The potassium ion efflux channel GORK plays a critical role in closing plant leaf stomata by releasing K+ from guard cells to reduce guard cell volume and turgor. The GUARD CELL OUTWARD-RECTIFYING K+ (GORK) channel is expressed in Arabidopsis guard cells and encodes a K+out channel. Voltage-dependent K+ channels, including GORK, contain three regions: an intracellular N-terminal region, a transmembrane region, and an intracellular C-terminal region (27–30). The transmembrane region is composed of six transmembrane helices (S1-S6), with S1-S4 forming the voltage sensing domain and S5 and S6 forming the pore region.

As a result, five different structures of GORK ranging from the transmembrane region to the C-terminal ANK (designated as GORKWT1–GORKWT5) were determined at resolutions of 3.16 to 3.27 Å. The five GORK structures showed N-terminally an almost uniform transmembrane domain (positions 50 to 313 from the initial Met), including the voltage-sensing domain and the ion selectivity filter. In contrast, the following cytosolic regions, i.e., C-linker (positions 314 to 364), CNBD (positions 365 to 490), CNBD–Ankyrin bridge (positions 491 to 542), and ANK (positions 543 to 722) show five distinct structures in almost twofold symmetry (C2 symmetry). Furthermore, overlaying GORKWT1 and GORKWT5, which had high resolutions of 3.17 and 3.16 Å, respectively, revealed that one of the C-linkers in each dimer was pushed upward by the CNBD in GORKWT1, as compared to GORKWT5. Closer inspection of the structure revealed that the difference of the degree of bending in the C-linker between Mol I and Mol II was small in GORKWT1 but greater in GORKWT5. Additionally, GORKWT1 displayed a C4-like C2 symmetry in the CNBD, whereas GORKWT5 showed a pronounced C2 symmetry. Furthermore, we found a structural difference in the short structure that lies between the CNBD and ANK domains, termed as CNBD–Ankyrin bridge containing residues 511 to 519. This region had an α-helical structure in GORKWT1, while in GORKWT5, it was entirely present in a nonhelical loop conformation. The CNBD–Ankyrin bridges of GORKWT1–GORKWT5 contain a mixture of α-helical and nonhelical structures, and these conformational changes appear to be centered around L516.

>MDYKDDDDKGRLRRRQEIIDHEEEESNDDVSSRRGKLSLAETFRWLDSSEHRRIETDGHNDYKYIIHPKNRWYKAWEMFILVWAIYSSLFTPMEFGFFRGLPERLFVLDIVGQIAFLVDIVLQFFVAYRDTQTYRTVYKPTRIAFRYLKSHFLMDFIGCFPWDLIYKASGKHELVRYLLWIRLFRVRKVVEFFQRLEKDTRINYLFTRILKLLFVEVYCTHTAACIFYYLATTLPPENEGYTWIGSLKLGDYSYENFREIDLWKRYTTALYFAIVTMATVGYGDIHAVNLREMIFVMIYVSFDMVLGAYLIGNITALIVKGSNTERFRDKMNDLISFMNRKKLGRDLRSQITGHVRLQYDSHYTDTVMLQDIPASIRAKIAQLLYLPYIKKVPLFKGCSTEFINQIVIRLHEEYFLPGEVITEQGNVVDHLYFVCEGLLEALVTKTDGSEESVTLLGPHTSFGDISIICNISQPFTVRVCELCHLLRLDKQSFSNILEIYFHDGRTILNNIMEEKESNDRIKKLESDIVIHIGKQEAELALKVNSAAFQGDFYQLKSLIRSGADPNKTDYDGRSPLHLAACRGYEDITLFLIQEGVDVNLKDKFGHTPLFEAVKAGQEGVIGLLVKEGASFNLEDSGNFLCTTVAKGDSDFLKRLLSSGMNPNSEDYDHRTPLHVAASEGLFLMAKMLVEAGASVISKDRWGNSPLDEARLCGNKKLIKLLEDVKNAQSSIYPSSLRELQEERIERRKCTVFPFHPQEAKEERSRKHGVVVWIPSNLEKLIVTAAKELGLSDGASFVLLSEDQGRITDIDMISDGHKLYMISDTTDQTHHHHHH[4x]>MSDENYRDIALAFLDESADSGTINAWVNEFAYQGFDPKRIVQLVKERGTAKGRDWKKDVKMMIVLNLVRGNKPEAMMKKMSEKGASIVANLISVYQLKEGNPGRDTITLSRVSAAFVPWTVQALRVLSESLPVSGTTMDAIAGVTYPRAMMHPSFAGIIDLDLPNGAGATIADAHGLFMIEFSKTINPSLR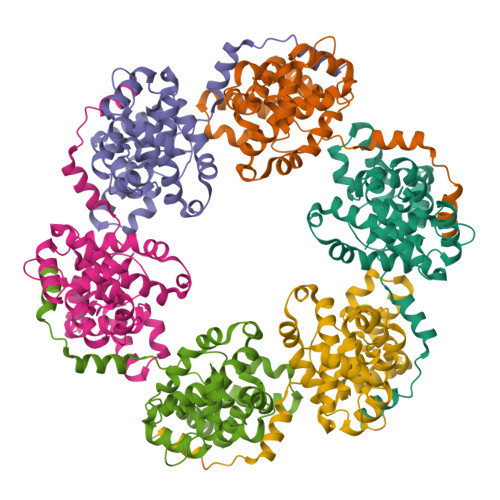TKQANEVAATFEKPNMAAMSGRFFTREDKKKLLIAVGIIDEDLVLASAVVRSAEKYRAKVGK[6x]>AQDMVSPPPPIADEPLTVNTGIYLIESYSLDDCAETFKVNAFLSLSWKDRRLAFDPVRSGVRVKTYEPEAIWIPEIRFVNVENARDADVVDISVSPDGTVQYLERFSARVLSPLDFRRYPFDSQTLHIYLIVRSVDTRNIVLAVDLEKVGKNDDVFLTGWDIESFTAVVKPANFALEDRLESKLDYQLRISRQYFSYIPNIILPMLFILFI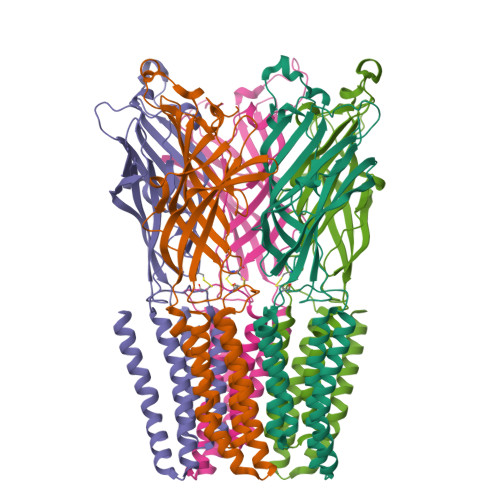SWTAFWSTSYEANVTLVVSTLIAHIAFNILVETCLPKTPYMTYTGAIIFMIYLFYFVAVIEVTVQHYLKVESQPARAASITRASRIAFPVVFLLANIILAFLFFGF[5x]>MGSSHHHHHHSSGLVPRGSHMSGSGSGSGTALTPSYLKDDDGRSLILRGFNTASSAKSAPDGMPQFTEADLAREYADMGTNFVRFLISWRSVEPAPGVYDQQYLDRVEDRVGWYAERGYKVMLDMHQDVYSGAITPEGNSGNGAGAIGNGAPAWATYMDGLPVEPQPRWELYYIQPGVMRAFDNFWNTTGKHPELVEHYAKAWRAVADRFADNDAVVAYDLMNAPFGGSLQGPAFEAGPLAAMYQRTTDAIRQVDQDTWVCVAPQAIGVNQGLPSGLTKIDDPRAGQQRIAYCPHLYPLPLDIGDGHEGLARTLTDVTIDAWRANTAHTARVLGDVPIILGEFGLDTTLPGARDYIERVYGTAREMGAGVSYWSSDPGPWGPYLP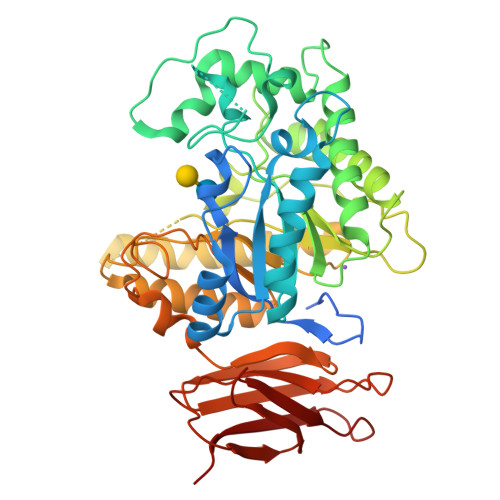DGTQTLLVDTLNKPYPRAVAGTPTEWSSTSDRLQLTIEPDAAITAPTEIYLPEAGFPGDVHVEGADVVGWDRQSRLLTVRTPADSGNVTVTVTPAA[2x]>[4x]MHHHHHHSTPSIVIASAARTAVGSFNGAFANTPAHELGATVISAVLERAGVAAGEVNEVILGQVLPAGEGQNPARQAAMKAGVPQEATAWGMNQLCGSGLRAVALGMQQIATGDASIIVAGGMESMSMAPHCAHLRGGVKMGDFKMIDTMIK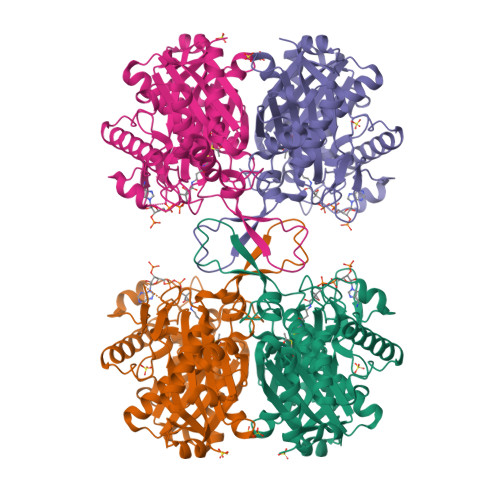DGLTDAFYGYHMGTTAENVAKQWQLSRDEQDAFAVASYNKAEAAQKDGRFKDEIVPFIVKGRKGDITVDADEEIRHGATLDSMAKLRPAFDKEGTVTAGNASGLNDGAAAALLMSEAEASRRGIQPLGRIVSWATVGVDPKVMGTGPIPASRKALERAGWKIGDLDLVEANEAFAAQACAVNKDLGWDPSIVNVNGGAIAIGHPIGASGARILNTLLFEMKRRGARKGLATLCIGGGMGVAMCIESL> MSVYPKALRDEYIMSKT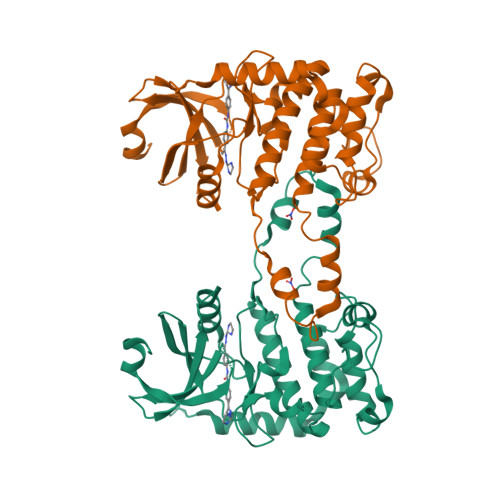LGSGACGEVKLAFERKTCKKVAIKIISKRKFAIGSAREADPALNVETEIEILKKLNHPCIIKIKNFFDAEDYYIVLELMEGGELFDKVVGNKRLKEATCKLYFYQMLLAVQYLHENGIIHRDLKPENVLLSSQEEDCLIKITDFGHSKILGETSLMRTLCGTPTYLAPEVLVSVGTAGYNRAVDCWSLGVILFICLSGYPPFSEHRTQVSLKDQITSGKYNFIPEVWAEVSEKALDLVKKLLVVDPKARFTTEEALRHPWLQDEDMKRKFQDLLSEENESTAKPQVLAQPSTSRKRPREGEAEGAE> GGSDFPSCRCVEQIIEKDEGPFYTHLGAGPNVAAIREIMEERFGQKGKAIRIERVIYTGKEGKSSQGCPIAKWVVRRSSSEEKLLCLVRERAGHTCEAAVIVILILVWEGIPLSLADKLYSELTETLRKYGTLTNRRCALNEERTCACQGLDPETCGASFSFGCSWSMYYNGCKFARSKIPRKFKLLGDDPKEEEKLESHLQNLSTLMAPTYKKLAPDAYNNQIEY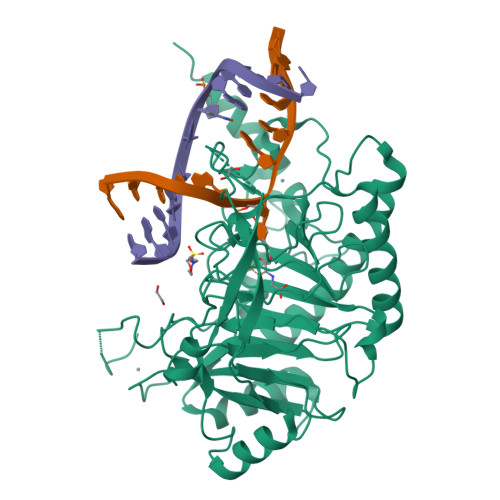EHRAPECRLGLKEGRPFSGVTACLDFCAHAHRDLHNMQNGSTLVCTLTREDNREFGGKPEDEQLHVLPLYKVSDVDEFGSVEAQEEKKRSGAIQVLSSFRRKVRMLAEPVKTCRQRKLEAKKAAAEKLSGGGGSGGGGSGGGGSDEVWSDSEQSFLDPDIGGVAVAPTHGSILIECAKRELHATTPLKNPNRNHPTRISLVFYQHKSMNEPKHGLALWEAKMAEKAREKEEECEKYG> MASSHHHHHHSSGLVPRGSSMGHNKKFDRSEHVYRNDSFLELIKDAVRFFSGTPVHSLPPPERFQGAGVYALYYTGHYSLYDEYSRINRLAYNLPIYVGKAVPAGWRQSRISDHETRAGSELSNRIREHGRNIAKTSNLDLCDFSCRFVIFEATGSDMISTVQAALIKIYKPLWNTVVDGFGNHTPGAGRFAQAKSDWDVIHPGREWAEKCTG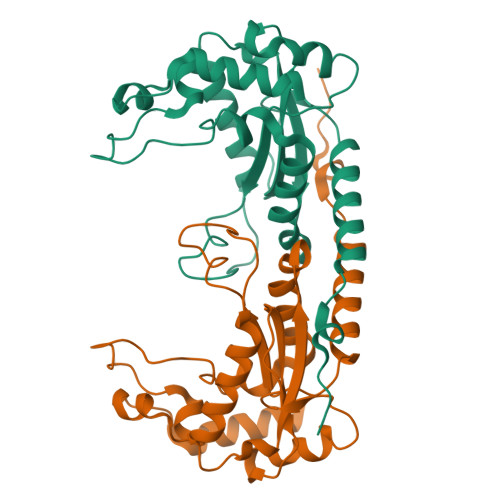VHSEPYFIEERIKQYFSKSNFT>MAATRQIQYTIPPREDYNKLSDEQKTRISEAFELFDSNKDGLLSYEEFRFVLRALGFDLPKQQTYDMLVRHGQRPANWPHDQECPPVYRQFNLATAQALAGTLIRQRDPRDELRRAFRLFDVDGKGMITEDDLRKVCQQVGNNIPDADIQAMIEEFDSNGKGGVDEDEFLRLMMSKK[2x];>[2x]GHMKPKRDLMADFTKWFVTGDGGIMEEFTEETLRHLLWDVWQRHQREEAERKRKAEEEESWRLAREHLTHRLQVKYFYRWREKARALAT;>[2x]GSSHHHHHHSQDLMASQHSPTPVKVPAAAANYTPATLDQDLRSQINSLLIKEGHVAKIQEHLLHHLHAHPSNWPTVVQNHALSLLRSGEVTSFPALLRRVVEDVRQDTALAPSSTTANGNGESTTTNGATNGKGATTNGNKGGVADLKPSLAVPQSVVEEALKVTRECLDQLCEIEEPLAA

The TREX-2 complex integrates mRNA nuclear export into the gene expression pathway and is based on a Sac3 scaffold to which Thp1, Sem1, Sus1, and Cdc31 bind. TREX-2 also binds the mRNA nuclear export factor, Mex67:Mtr2, through the Sac3 N-terminal region (Sac3N). Whereas protein transport is generally facilitated by karyopherin-β family proteins, mRNA export in yeast is mediated primarily by the Mex67:Mtr2 complex or in metazoans by NXF1:NXT1 (Segref et al., 1997; Braun et al., 2001). Mex67 is a modular protein containing four domains: RNA-recognition motif (RRM), leucine-rich repeat (LRR), nuclear transport factor 2-like (NTF2L), and ubiquitin-associated (UBA).

Bacterially expressed ctSus1 formed a tripartite complex with ctSac3CID and ctCdc31, and the crystal structure of this complex confirmed that the appropriate Chaetomium genes had been identified. Crystalline plates of the C. thermophilum Sac3CID:Sus1:Cdc31 complex were obtained that diffracted to 3.3 Å resolution, and molecular replacement produced clear and well-defined electron density maps. After refinement, the model had a Rwork/Rfree value of 21.8%/27.7% and excellent geometry. Although its overall fold was similar to its S. cerevisiae homolog, the C. thermophilum Sac3CID:Cdc31:Sus1 complex had only a single Sus1 chain, whereas in the corresponding S. cerevisiae and GANP structures Sac3 bound two Sus1 chains, although only one of these chains appeared to be important functionally (Jani et al., 2009, 2012). In the C. thermophilum complex, the Sac3 helix also had a “kink” following residue 1,137, possibly as a consequence of the greater distance between the Cdc31 and Sus1 chains. The overall folds of ctCdc31 and ctSus1 were strongly conserved with their S. cerevisiae counterparts, with root-mean-square deviations (RMSDs) of 2.56 Å over 88 C-α atoms for Sus1 and 3.10 Å over 144 C-α atoms for Cdc31. The helical elements of the folds of both proteins were fully conserved, with differences concentrated in the loops joining the helices. Density for ctSus1 residues 99–139, as well as its substantially longer N/C-terminal extensions, was not present, consistent with these regions being disordered. Importantly, the extensive interaction interfaces between Sac3 and both Cdc31 and Sus1 were preserved. For example, ctSac3 Trp1161 was analogous to scSac3 Trp802, where it is a central feature of the Sac3-Cdc31 interaction and is buried in a hydrophobic cavity in the Cdc31 C-terminal domain.>[2x]GHMAKTYDYLFKLLLIGDSGVGKTCVLFRFSEDAFNSTFISTIGIDFKIRTIELDGKRIKLQIWDTAGQERFRTITTAYYRGAMGIMLVYDITNEKSFDNIRNWIRNIEEHASADVEKMILGNKCDVNDKRQVSKERGEKLALDYGIKFMETSAKANINVENAFFTLARDIKAKMDKKLEGNSPQG;>[4x]GPEKGSEFLKEELHRAQKELKLKDEECERLSKVREQLEQ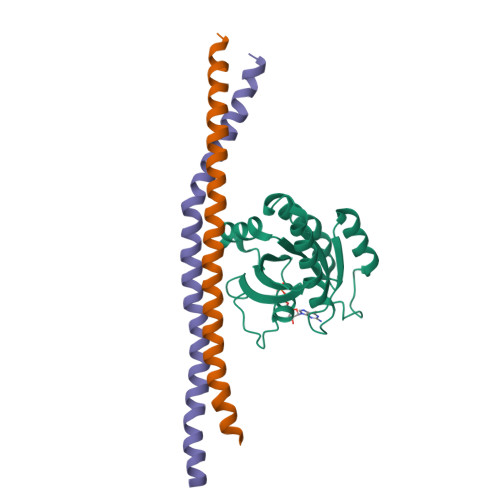ELEELTASLFEEAHKMVREANMKQAASEKQLKEARGKIDMLQAEV> MFEINPVNNRIQDLTERSDVLRGYLDYDAKKERLEEVNAELEQPDVWNEPERAQALGKERSSLEAVVDTLDQMKQGLEDVSGLLELAVEADDEETFNEAVAELDALEEKLAQLEFRRMFSGEYDSADCYLDIQAGSGGTEAQDWASMLERMYLRWAESRGFKTEIIEESEGEVAGIKSVTIKISGDYAYGWLRTETGVHRLVRKSPFDSGGRRHTSFSSAFVYPEVDDDIDIEINPADLRID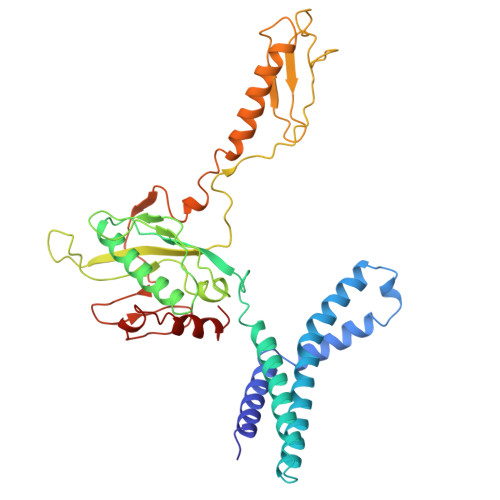VYRASGAGGQHVNRTESAVRITHIPTGIVTQCQNDRSQHKNKDQAMKQMKAKLYEVEMQKKNAEKQAMEDNKSDIGWGSQIRSYVLDDSRIKDLRTGVETRNTQAVLDGSLDQFIEASLKAGL> GSKRDHHQFQGRLSNHGTSSSSSSISKDKMMMVKKEEDGGGNMDDELLAVLGYKVRSSEMAEVALKLEQLETMMSNVQEDGLSHLATDTVHYNPSELYSWLDNMLSELNPPPLPASSNGLDPVLPSPEICGFPASDYDLKVIPGNAIYQFPAIDSSSSSNNQNKRLKSCSSPDSMVTSTSTGTQIGGVIGTTVTTTTTTTTAAGESTRSVILVDSQENGVRLVHALMACAEAIQQNNLTLAEA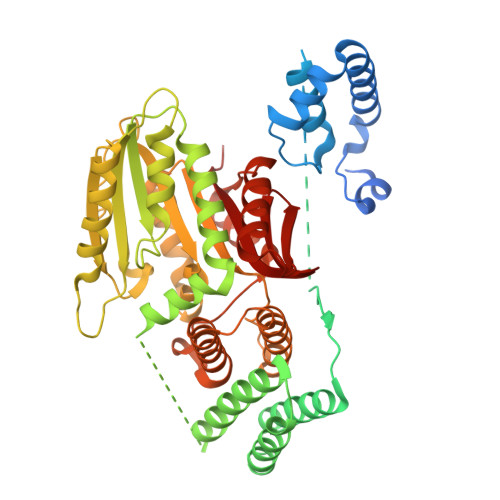LVKQIGCLAVSQAGAMRKVATYFAEALARRIYRLSPPQNQIDHCLSDTLQMHFYETCPYLKFAHFTANQAILEAFEGKKRVHVIDFSMNQGLQWPALMQALALREGGPPTFRLTGIGPPAPDNSDHLHEVGCKLAQLAEAIHVEFEYRGFVANSLADLDASMLELRPSDTEAVAVNSVFELHKLLGRPGGIEKVLGVVKQIKPVIFTVVEQESNHNGPVFLDRFTESLHYYSTLFDSLEGVPNSQDKVMSEVYLGKQICNLVACEGPDRVERHETLSQWGNRFGSSGLAPAHLGSNAFKQASMLLSVFNSGQGYRVEESNGCLMLGWHTRPLITTSAWKLSTAAY We present crystal structures of a new NAD+-binding riboswitch termed NAD+-II, bound to nicotinamide mononucleotide (NMN), nicotinamide adenine dinucleotide (NAD+) and nicotinamide riboside (NR). The RNA structure comprises a number of structural features including three helices, one of which forms a triple helix by interacting with an A5 strand in its minor-groove, and another formed from a long-range pseudoknot. Unusually the riboswitch binds two molecules of ligand, bound at distinct, non-overlapping sites in the RNA. Binding occurs primarily through the nicotinamide moiety of each ligand, held by specific hydrogen bonding and stacking interactions with the pyridyl ring.

The RNA structure of the riboswitch bound to NAD+ superimposes very well with that bound to NMN, with an RMSD of 0.582 Å. The structure contains two bound NAD+ ligands, with their nicotinamide moieties bound essentially identically to the NMN in the two-strand structure discussed above. The electron density map for the nicotinamide moiety and diphosphate bound at site 1 is very good, but poorer for the adenosine moiety. But nevertheless, the adenine predominantly locates in a pocket at the end of the P1a helix. The adenine nucleobase is stacked on that of C30 at the end of P1a, and within the pocket its N6 donates a hydrogen bond to N1 of A18. In effect the NAD+ adenine and A18 form a trans Hoogsteen-Watson-Crick base pair stacked on the end of the P1a helix. The NAD+ ligand binds to the riboswitch in an extended conformation (the nicotinamide and adenine moieties are separated by 14 Å), on the major groove side of the 2N4 region, with nicotinamide and adenine ends located in well-separated cavities in the RNA. The positions of the nicotinamide moiety and diphosphate for the ligand bound at site 2 are well defined, but the position of the adenine nucleoside (particularly the ribose) is poorly defined. The trajectory of the diphosphates indicates that the adenine moiety emerges from the PK major groove, but the adenine appears to make no interactions with the RNA.

>CGCGGCGUUGCGUCCGAAAGUCUAAACAGACACGGCCGCUUAAAAACAAAAGGAGA[2x]> GPLGSPEFPGAFRTQKPSLNTVNVVGSSMGSGGVFTIDGKIKCVT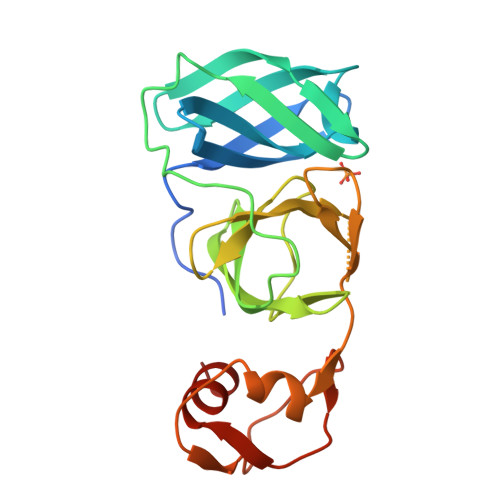AAHVLTGNSARVSGVGFNQMLDFDVKGDFAIADCPNWQGVAPKAQFCEDGWTGRAYWLTSSGVEPGVIGNGFAFCFTACGDSGSPVITEAGELVGVHTGSNKQGGGIVTRPSGQFCNVKPIKLSELSEFFAGPKVPLGDVKIGSHIIKDTCEVPSDLCALLAAKPELE>GDAYAQWLADGGPSSGRPPPSG[3x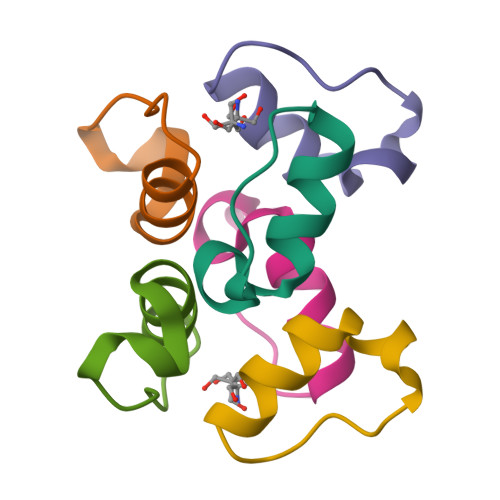]>ETELRPRGRSLVIISTLDGRIAALDPENHGKKQWDLDVGSGSLVSSSLSKPEVFGNKMIIPSLDGALFQWDQDRESMETVPFTVESLLESSYKFGDDVVLVGGKSLTTYGLSAYSGKVRYICSALGCRQWDSDEMEQEEDILLLQRTQKTVRAVGPRSGNEKWNFSVGHFELRYIPDMETRAGFIESTFKPNENTEESKIISDVEEQEAAIMDIVIKVSVADWKVMAFSKKGGHLEWEYQFCTPIASAWLLKDGKVIPISLFDDTSYTSNDDVLEDEEDIVEAARGATENSVYLGMYRGQLYLQSSVRISEKFPSSPKALESVTN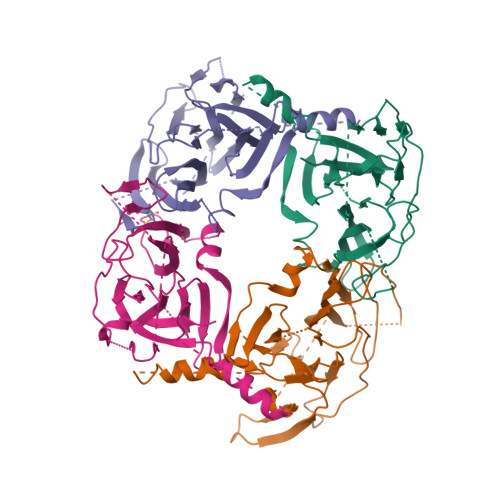E[4x]Antifreeze proteins (AFPs) inhibit ice growth by adsorbing onto specific ice planes. To probe the molecular mechanisms responsible for AFP activity, we here characterized the antifreeze activity and crystal structure of TisAFP7 from the snow mold fungus Typhula ishikariensis. TisAFP7 exhibited intermediate activity, with the ability to bind the basal plane, compared with a hyperactive isoform TisAFP8 and a moderately active isoform TisAFP6. The structure is dominated by a right-handed β-helical domain, a typical DUF3494 structure.

The crystal structure of TisAFP7 T20Y was determined at 1.72 Å resolution. The crystal was isomorphous with the wild-type crystal, and the final structure was refined with R-factor of 0.208 and Free R of 0.246, containing 446 residues and 554 solvent molecules. Indeed, both substitutions resulted in a reduced TH activity (0.4 °C at 0.25 mM T20Y mutant and 0.45 °C at 0.27 mM A214Y mutant), equivalent to a 60% and 50% reduction from wild-type TisAFP7, accordingly. Panels 1 and 2, the T20Y mutant covered only the perimeter zone of the hemisphere, corresponding to the secondary prism planes. The reduced coverage of ice planes by the T20Y mutant indicated lost ice-binding affinity for the basal, primary prism, and some pyramidal planes. The water network of TisAFP7 was less extensive than that of TisAFP8. This prompted us to propose that the antifreeze activity of TisAFPs, typically reflecting the affinity toward the ice basal plane, is correlated with the water coverage on IBS via the extended network of water molecules, as observed in the current study. In the mutant, the bound water molecules near residue 20 were removed by introducing the side chain of Tyr, thus truncating the zigzag pattern.

>[2x]AGPTAVPLGTAGNYAILASYAVSTVPQSAITGAVGISPAAGTFLTGFSLTMSGTGTFSTSTQVTGQLTAADYGTPTPSILTTAIGDMGTAYTNGATRSGPDFLEIYTGALGGTTLLPGLYKWTSSVGASADFTISGTSTDTWIFQIDGTLGLAAGKKITLAGGAQAKNIIWVVAGAVSIEAGAQFEGVILAKTAVTLKTGSSLNGRILAQTSVALQSATVVQK> ENLYFQGHMDNVDELRKIENKSSFVSADNMPEYVKGAFISMQDERFYNHHGFDLKGTTRALFSTISDRDVQGGSTITQQVVKNYFYDNDRSFTRKVKELFVAHRVEKQYNKNEILSFYLNNIYFGDNQYTLEGAANHYFGTTVNKNSTTMSHITVLQSAILASKVNAPSVYNINNMSENFTQRVSTNLEKMKQQNYINETQYQQAMSQLN

PG is synthesized from its precursor lipid II (GlcNAc-MurNAc(pentapeptide)-undecaprenyl pyrophosphate) by the concerted action of membrane-bound enzymes containing the PG glycosyltransferase (PGT) and transpeptidase (TP) domains (Sauvage et al., 2008, Lovering et al., 2012). The PGT module is found in two different families of PG synthases; as a single domain in monofunctional glycosyltransferases (MGTs) and as the N-terminal domain of the bifunctional class A penicillin-binding proteins (PBPs). The PGT domain adopts an all α-helical globular fold with an extended groove that divides this domain into two subdomains—a large head subdomain containing features similar to the bacteriophage λ-lysozyme and a small jaw subdomain containing features specific to the glycosyltransferase family 51 (GT51). The flap region adopts an α-helix-loop structure and serves as a steric barrier to physically separate the PGT enzymatic cavity into two substrate-binding sites—a donor site for the lipid-bound growing glycan chain and an acceptor site for the lipid II.

The difference map produced by the phenix.polder tool in PHENIX shows for the first time a complete C25 moenocinol lipid tail of MoeADON modelled into the structure. Additional electron density was observed in the groove accommodating ring A of MoeADON which is consistent with a non-ionic surfactant: glyceryl monolaurate used during cell lysis procedure. The polar end of glyceryl monolaurate makes strong hydrogen bond interactions with the side chains of Asp184, Tyr196 and the backbone atoms of Pro226, Ser227, Val228, Tyr229 and Asn230. Our analyses also revealed a large positive electron density extending from the bound phosphate ion at the base of the jaw subdomain (His107 to Leu112), along the external surface, connecting to an additional area of positive electron density at the mouth of a deep pocket just below the catalytic site. This deep pocket is surrounded by the conserved residues in what we now define as motif I (Asp101, His107, Gly109, Asp111), motif II (Gln129, Gly130, Gly131, Ser132, Thr133, Gln136) and motif III (Lys153), suggesting its functional significance. The difference density from the polder map was sufficient to fit the A and B rings of MoeA at the mouth of the deep pocket and ring F connecting the bound phosphate ion at the base of the jaw subdomain. Saccharide rings C, D, E and the C25 moenocinol lipid tail could not be modelled due to a lack of significant difference density. The overall electron density suggested that sections of a second MoeA molecule (i.e. MoeAJAW) bound to the jaw subdomain could be modelled at this site. The ring B of MoeAJAW forms hydrogen bonds with the side chains of Asp101, Gln136, the backbone carbonyl oxygen atom of Phe110 and the water molecules in the pocket.> SHSTAETTLDSFFSRAGLVGEIDLPLEGTTNPNGYANWDIDITGYAQMRRKVELFTYMRFDAEFTFVACTPTGQVVPQLLQYMFVPPGAPKPDSRESLAWQTATNPSVFVKLSDPPAQVSVPFMSPASAYQWFYDGYPTFGEHKQEKDLEYGACPNNMMGTFSVRTVGTSKSKYPLVIRIYMRMKHVRAWIPRPMRNQNYLFKANPNYAGNFIKPTGASRTAITT;> LTIGNSTITTQEAANIIVGYGEWPSYCSDSDATAVDKPTRPDVSVNRFYTLDTKLWEKSSKGWYWKFPDVLTETGVFGQNAQFHYLYRSGFCIHVQCNASKFHQGALLVAVLPEYVIGTVAGGTGTEDSHPPYKQTQPGADGFELQHPYVLDAGIPISQLTVCPHQWINLRTNNCATIIVPYINALPFDSALNHCNFGLLVVPISPLDYDQGATPVIPITITLAPMCSEFAGLRQ;> GFPTELKPGTNQFLTTDDGVSAPILPNFHPTPCIHIPGEVRNLLELCQVETILEVNNVPTNATSLMERLRFPVSAQAGKGELCAVFRADPGRSGPWQSTLLGQLCGYYTQWSGSLEVTFMFTGSFMATGKMLIAYTPPGGPLPKDRATAMLGTHVIWDFGLQSSVTLVIPWISNTHYRAHARDGVFDYYTTGLVSIWYQTNYVVPIGAPNTAYIIALAAAQKNFTMQLCKDASDIL

Enteroviruses particles are composed of single-strand RNA (virion RNA) genomes encapsulated by an icosahedral capsid of ~30 nm in diameter. In this study, we genetically perturb this equilibrium in a non-enveloped virus, enterovirus A71 to determine its structural basis. We isolate a single-point mutation variant with increased particle thermotolerance and decreased efficiency of cell entry. Using cryo-electron microscopy and molecular dynamics simulations, we determine that the thermostable native particles have acquired an expanded conformation that results in a significant increase in protein dynamics.

Particle conversion from N to empty capsids (E) follows a predetermined protein unfolding process that can be mimicked by incubating the purified N particles at high temperature. Accordingly, native particles of the WT and K162E were heated at 52 °C for 1 h to convert them to inactivated A-particle or empty E particles. Heat-inactivated particles were reconstructed using 2D class averaging and icosahedral symmetry-based 3D reconstruction. Particles then were classified according to whether they had Coulomb potential at the center of the particle. A-particles showed density, but empty particles did not. The WT A- and E-particles were resolved to a resolution of 8.0 and 14 Å, respectively. Even at this relatively low resolution, the A-particle matches previously described structures (EMDB ID: 5465), with a cross-correlation score of 0.918. The A-particle capsid proteins expand outward, the virion RNA genome becomes reorganized, the N-terminus of capsid protein VP1 is exposed on the surface of the particle, and VP4 is lost.> ANPYERGPDPTQASLEASRGPFPVSEERVSSPVSGFGGGTIYYPQENNTYGAVAISPGYTATQSSVAWLGERIASHGFVVITIDTNTTLDQPDSRADQLEAALDHMVDGASSTVRSRIDRNRLAVMGHSMGGGGTLRLASRRPDLKAAIPLTPWHLNKSWSNVQVPTLIIGAENDTVAPVALHAEPSYTSIPTSTRKAYLELNGASHFAPSVANATIGMYGVAWLKRFVDEDTRYTRFLCPGPRTGLFSD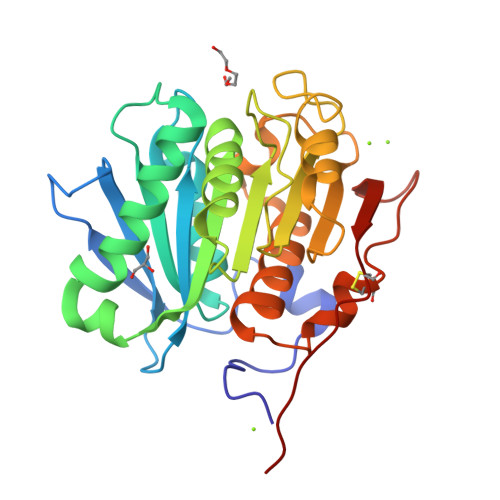VEEYRSTCPFLEHHHHHH> GSEGQ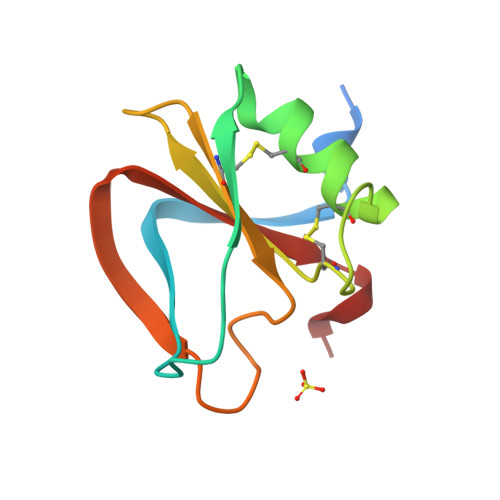KKRRNTLHEFKKSAKTTLTKEDPLLKIKTKKVNSADECANRCIRNRGFTFTCKAFVFDKSRKRCYWYPFNSMSSGVKKGFGHEFDLYENKDYIR> MAAKSDGRLKMKKSSDVAFTPLQNSDHSGSVQGLAPGLPSGSGAEDEEAAGGGCCPDGGGCSRCCCCCAGSGGSAGSGGSGGVAGPGGGGAGSAALCLRLGREQRRYSLWDCLWILAAVAVYFADVGTDVWLAVDYYLRGQRWWFGLTLFFVVLGSLSVQVFSFRWFVHDFSTEDSATAAAASSCPQPGADCKTVVGGGSAAGEGEARPSTPQRQASNASKSNIAAANSGSNSSGATRASGKHRSASCSFCIWLLQSLIHILQLGQIWRYFHTIYLGIRSRQSGENDRWRFYWKMVYEYADVSMLHLLATFLESAPQLVLQLCIIVQTHSLQALQGFTAAASLVSLAWALASYQKALRDSRDDKKPISYMAVIIQFCWHFFTIAARVITFALFASVFQLYFGIFIVLHWCIMTFWIVHCETEFCITKWEEIVFDMVVGIIYIFSWFNVKEGRTRCRLFIYYFVILLENTAL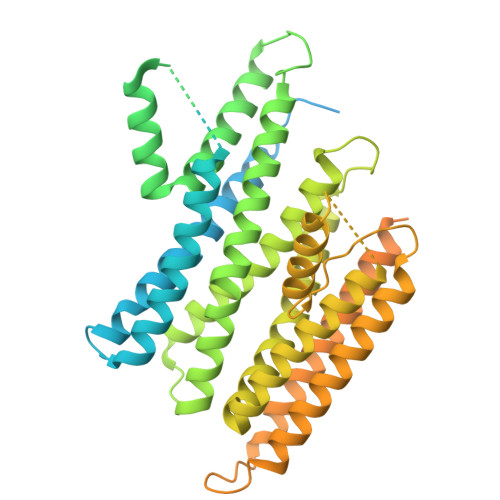SALWYLYKAPQIADAFAIPALCVVFSSFLTGVVFMLMYYAFFHPNGPRFGQSPSCACEDPAAAFTLPPDVATSTLRSISNNRSVVSDRDQKFAERDGCVPVFQVRPTAPSTPSSRPPRIEESVIKIDLFRNRYPAWERHVLDRSLRKAILAFECSPSPPRLQYKDDALIQERLEYETTL> HHHHHHSDQMVKYFLGQSVLRSSWDQVFAAFWQRYPNPYSKHVLTEDIVHREVTPDQKLLSRRLLTKTNRMPRWAERLFPANVAHSVYVLEDSIVDPQNQTMTTFTWNINHARLMVVEERSVYSVNSDNSGWTEIRREAWVSSSLFGVSRAVQEFGLARFKSNVTKTMKGFEY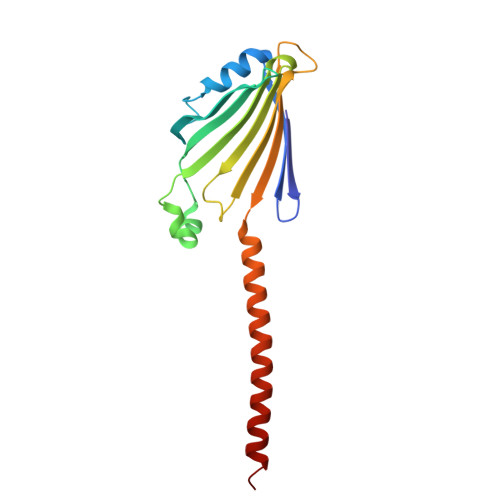ILAKLQGEA5-(dimethylamino)-~{N}-[6-[(2~{R},3~{R},4~{S},5~{R})-3-(hydroxymethyl)-4,5-bis(oxidanyl)piperidin-2-yl]hexyl]naphthalene-1-sulfonamide 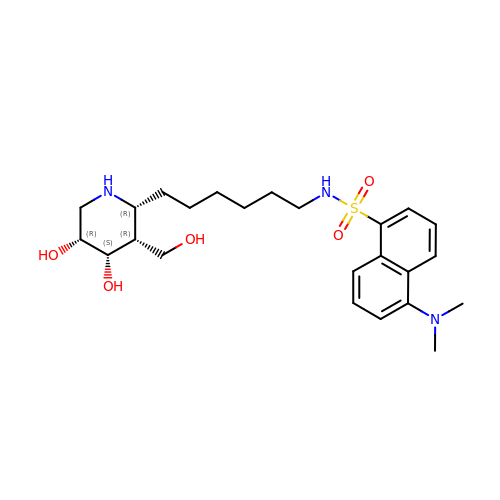| C24 H37 N3 O5 S | YUUSOYGEJQMOTK-IKJKNFHUSA-N6-(4-fluorophenyl)quinolin-8-ol | C15 H10 F N O 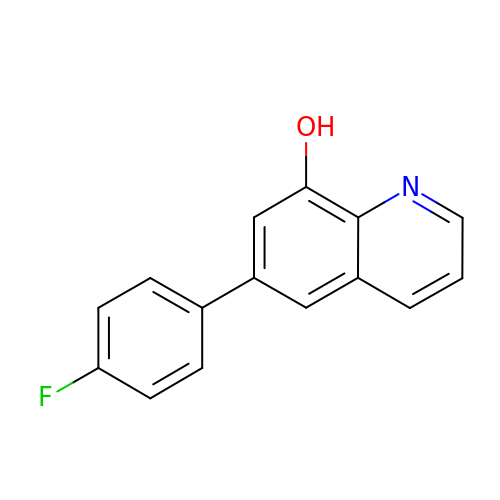| FTIUFDNWKCYJNH-UHFFFAOYSA-N>ACDYTCGSNCYSSSDVSTAQAAGYKLHEDGETVGSNSYPHEFRNWNGFDFSVSSPYY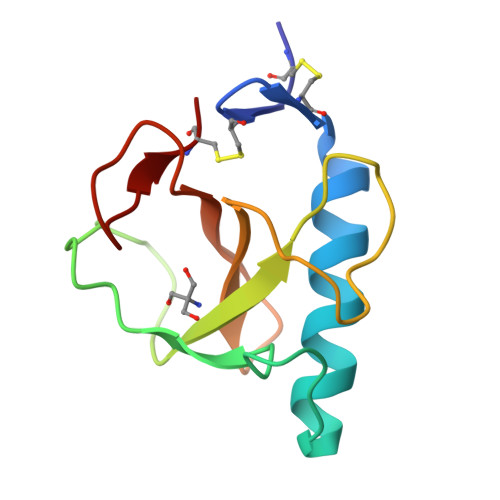EYPILSSGDVYSGGSPGADRVVFNENNQLAGVITHTGASGNNFVECT[3x]~{N}-(furan-2-ylmethyl)-2-methyl-furan-3-carboxamide | C11 H11 N O3 | 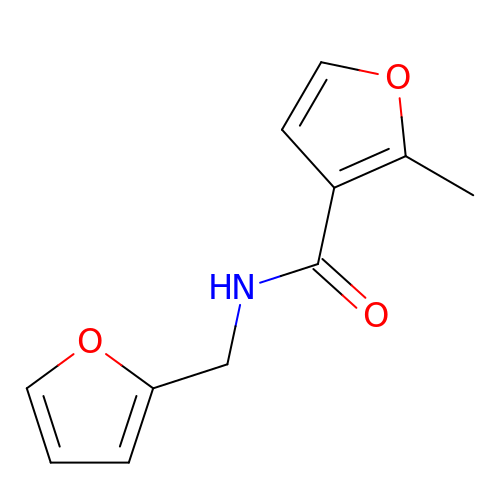ZSEHNDARAQYZIE-UHFFFAOYSA-N>[2x]LDKLHVTSTRPQYVRIKNWGSGEILHDTLHHKATSDFTCKSKSCLGSIMNPKSLTRGPRDKPTPLEELLPHAIEFINQYYGSFKEAKIEEHLARLEAVTKEIETTGTYQLTLDELIFATKMAWRNAPRCIGRIQWSNLQVFDARNCSTAQEMFQHICRHILYATNNGNIRSAITVFPQRSDGKHDFRLWNSQLIRYAG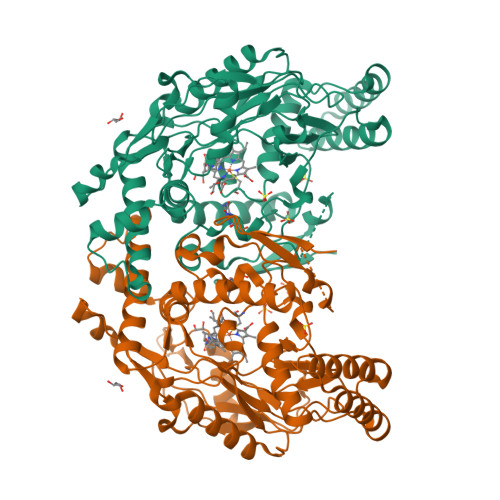YQMPDGTIRGDAATLEFTQLCIDLGWKPRYGRFDVLPLVLQADGQDPEVFEIPPDLVLEVTMEHPKYEWFQELGLKWYALPAVANMLLEVGGLEFPACPFNGWYMGTEIGVRDFCDTQRYNILEEVGRRMGLETHTLASLWKDRAVTEINVAVLHSFQKQNVTIMDHHTASESFMKHMQNEYRARGGCPADWIWLVPPVSGSITPVFHQEMLNYVLSPFYYYQIEPWKTHIWQNE>[4x]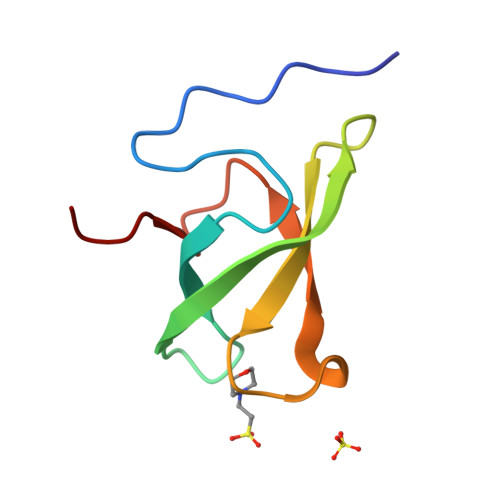GSHMPPNRPGITFEIGARLEALDYLQKWYPSRIEKIDYEEGKMLVHFERWSHRYDEWIYWDSNRLRPLER> ARSTNTFNYATYHTLDEIYDFMDLLVAEHPQLVSKLQIGRSYEGRPIYVLKFSTGGSNRPAIWIDLGIHSREWITQATGVWFAKKFTEDYGQDPSFTAILDSMDIFLEIVTNPDGFAFTHSQNRLWRKTRSVTSSSLCVGVDANRNWDAGFGKAGASSSPCSETYHGKYANSEVEVKSIVDFVKDHGNFKAFLSIHSYSQLLLYPYGYTTQSIPDKTELNQVAKSAVAALKSLYGTSYKYGSIITTIYQASGGSIDWSYNQGIKYSFTFELRDTGRYGFL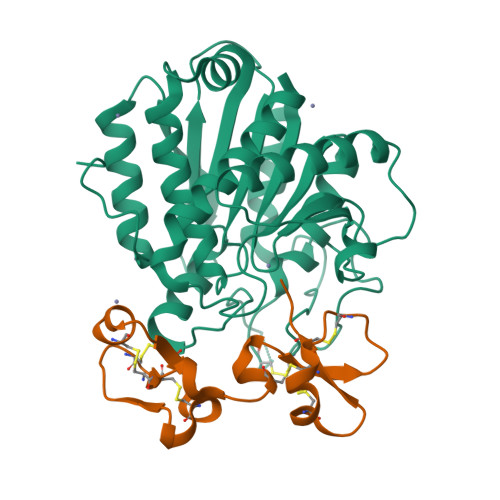LPASQIIPTAQETWLGVLTIMEHTVNNLY;> NECVSKGFGCLPQSDCPQEARLSYGGCSTVCCDLSKLTGCKGKGGECNPLDRQCKELQAESASCGKGQKCCVWLH> MSNSITVRARGVNGQESVSLQVGGTTVQTWTLTTAMQD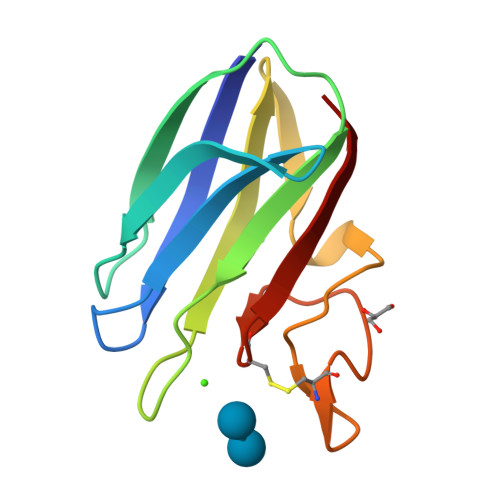YTASTSLTGEIRVAFTNDATGRDVQVDYIVVNGQTRQAENQSVNTGVWANNQCGGSGNSEWLHCNGYISFGNVS> MSRSRPELGDWSSPAELAELQRSQLPRVLAQALRSPFYAARYRGTTPPRTADDFAGVEVTAKQDLRDQYPFGMLAVGREHLATYHESSGTAGEPTASYYTEEDWTDLAERFARKWTGIHPSDTFLVRTPYGLVITGHLAQAAGRLRGATVVPGDARSLATPLSRMVRVLKTLDVTLTWCNPTEITMLAAAAKAAGLRPDQDFPHLRAMFTAAEPLTEVRRRRLSEIWGGIPVVEEYGSTETGTIAGQCPE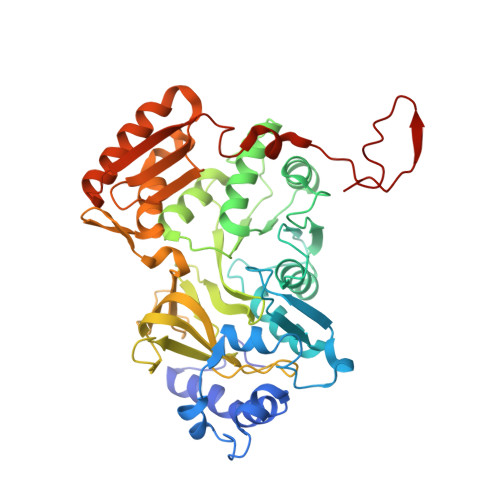GRMHLWADRAIFEVYDPRTGTLSEAGRGQMVVTPLYRDAMPLLRYNLADDVEVSTDPCGCGWLLPTVTVLGRAGTGHRIGPATVTQQRLEELVFSLPAAYEVMFWRAKAHPDVLELEFEAPEPVRQRAVKELGAALDRELGVPHRITGLAPGTLVPAEALTAQRDILKARYLFAEDEDWDKAVMYF> AECSVDIQGNDQMQFNTNAITVDKSCKQFTVNLSHPGNLPKNVMGHNWVLSTAADMQGVVTDGMASG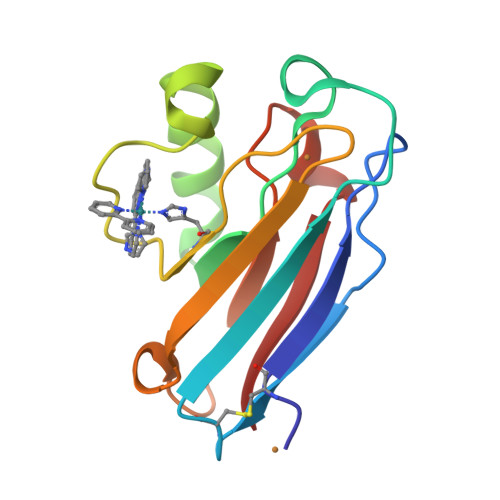LDKDYLKPDDSRVIAHTKLIGSGEKDSVTFDVSKLKEGEQYMFFCTFPGHSALMKGTLTLK> MISDAMRLIQVALQRYILEFEPELGLSQVVIIENIAMAEELGG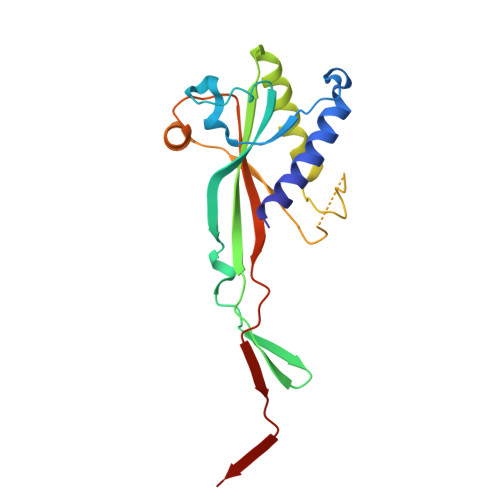QNNQINGHVVMSLVNLQEETTLKNSPHYRLDNGRTIYQNPPVNLNLFILFSALHNQYETSLRLLSRVVEFFQWQKELSFTTTPGIGGISRDLRILPDLYSLTFEQLNHLWGALGGKQVPFVLYRARILSLEAPKRQAEGSTITEIYINE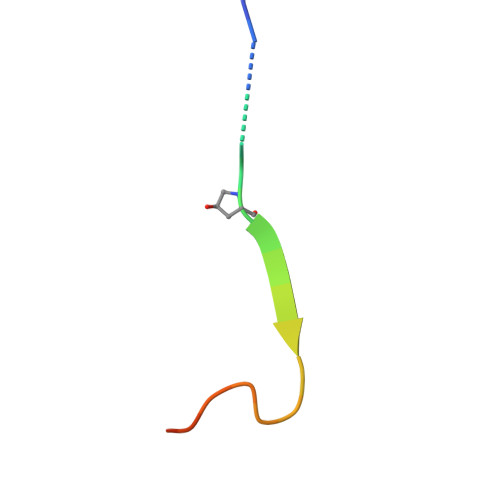> GLPGTAGLPGMKGHRGFSGLDGY>[2x]MASSNLIKQLQERGLVAQVTDEEALAERLAQGPIALYCGFDPTADSLHLGHLVPLLCLKRFQQAGHKPVALVGGATGLIGDPSFKAAERKLNTEETVQEWVDKIRKQVAPFLDFDCGENSAIAANNYDWFGNMNVLTFLRDIGKHFSVNQMINKEAVKQRLNREDQGISFTEFSYNLLQGYDFACLNKQYGVVLQIGGSDQWGNITSGIDLTRRLHQNQVFGLTVPLITKADGTKFGKTEGGAVWLDPKKTSPYKFYQFWINTADADVYRFLKFFTFMSIEEINALEEEDKNSGKAPRAQYVLAEQVTRLVHGEEGLQAAKRITECLFSGSLSALSEADFEQLAQDGVPMVEMEKGADLMQALVDSELQPSRGQARKTIASNAITINGEKQSDPEYFFKEEERLFGRFTLLRRGKKNYCLICWK

The aminoacyl-tRNA synthetases (aaRSs) are essential enzymes playing a central role in the translation of the genetic code and hence constitute a viable target for the development of antibiotics. Based on the structure of the catalytic site, two distinct classes of tRNA synthetases can be discerned. Both classes activate an amino acid in forming the respective aminoacyl-adenylate (aa-AMP) as natural reaction intermediates. In view of their resemblance and irrespective of the class, aminoacyl-sulfamoyl adenosine (aaSA) derivatives are well-known high-affinity aaRS inhibitors, but they lack antibacterial activity due to their low uptake potential. Structural analysis showed the flipped 2-hydroxymethyl-1,3-dideazaadenine base is partially mimicking the interactions of adenine within both series of aaRS enzymes.

The compound was unambiguously built inside the active site of tRNA synthetase according to the electron density map, which confirmed the conformation of the flipped base. With the present modification, in most cases, the amine group occupies the place where the N3 of adenine is normally residing and mimics its interaction with the protein. In the case of class I aaRSs, only two polar interactions with the base are consistently observed for the different aaRS:aaSA complex structures, mediated by the interaction of the protein backbone atoms with the N1 and N6 atoms of adenine. In this work, the flipped base loses part of these important interactions, providing a good rationale for their lower activity compared with aaSA. In addition, the hydroxymethyl group of the base makes H-bonds with backbone atoms of Val583 in LeuRS or Ile228 in TyrRS, respectively. However, in the case of SerRS, the base moiety adopts the syn-conformation relative to the ribose defined by the torsion angle (O4′-C1′-N7-C8) of −124°, while the base bound in the active site of class I LeuRS and TyrRS and class II AspRS remains in the anti-conformation. In the case of the class I-targeting compounds, low-nanomolar Kiapp were obtained for the 7HMDDA derivatives 32e–f and 1.2 µM for 32b targeting TyrRS. While these values reflect high affinity for the target enzymes, the inhibition is 5 to 420-fold lower compared to that with the original aaSA analogue. While TyrS7HMDDA was about 400 times less inhibitory compared to TyrSA, the 3DA and the uracil analogue only gave 10-fold and 15-fold reductions in activity, respectively, while the cytosine congener also suffered a 400-fold decreased inhibitory activity.2,4-dibromo-6-({[(2-chlorophenyl)carbonyl]amino}methyl)phenyl 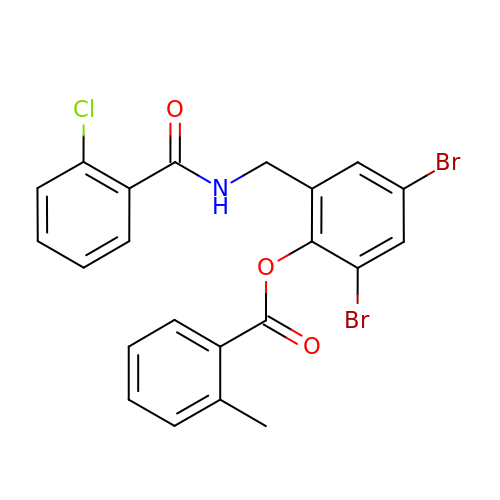2-methylbenzoate | C22 H16 Br2 Cl N O3 | ZXLLGHNQLPHULK-UHFFFAOYSA-N> MALTKAEMSEYLFDKLGLSKRDAKELVELFFEEIRRALENGEQVKLSGFGNFDLRDKNQRPGRNPKTGEDIPITARRVVTFRPGQKLKSRVENASPKDE;> MTKSELIERLATQQSHIPAKTVEDA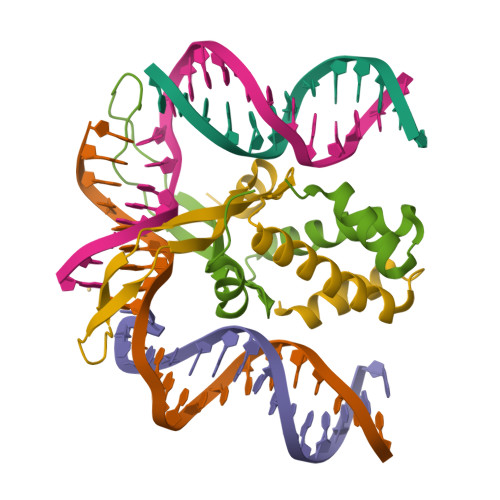VKEMLEHMASTLAQGERIEIRGFGSFSLHYRAPRTGRNPKTGDKVELEGKYVPHFKPGKELRDRANIYG DyPs (dye-decolorizing peroxidases) (EC 1.11.1.19) represent a new family of haem peroxidases widespread in bacteria, archaea, fungi and other micro-organisms. In the present study, we expressed A. auricula-judae DyP in E. coli, solved the crystal structure of the recombinant enzyme and several site-directed variants, and used PELE (Protein Energy Landscape Exploration) to describe the binding of its typical substrate RB19. The DyP structure is formed by two domains, each of them including an antiparallel four-stranded large β-sheet and two or three helices resulting in a ferredoxin-like fold (plus two additional β-strands). In spite of the obvious similarity between the two domains, only the C-terminal domain harbours a haem cofactor.

Among them, Tyr-147, Tyr337 and Trp-377 are solvent-exposed, but Trp-105 and Tyr-285 are buried into the protein making their interaction with the dye substrate more difficult. Aromatic residues were changed to serine in the simple W377S, Y147S and Y337S variants (the latter with low refolding yield). Moreover, most of the variants show crystal structures largely superimposable with that of WT DyP, except for the mutated residues. In contrast, similar Tyr-337 and Tyr-147 variants (and the double Y147F/Y337F variant) only slightly affected substrate oxidation, and did not remove the high-turnover site. However, this does not seem to be due to modification of Tyr-337 (or contiguous Tyr-147) since the enzyme activity was practically unaffected after site-directed mutagenesis of these two residues. Among the 65 DyP sequences compared, 58 include a tryptophan residue homologous with Trp-377, and 48 include a tyrosine residue homologous with Tyr-337 (whereas the neighbour Tyr-147 is only conserved in 14 sequences).

>MATSLNTIDIQGDILVGMHKQKQLFYFFAINDPATFKTHLASDIAPVVASVTQLSNVATQPLVALNIAFSNTGLLALGVTDNLGDSLFANGQAKDATSFKESTSSWVPQFAGTGIHGVIILASDTTDLIDQQVASIESTFGSSISKLSSLSASIRPGNEAGHEMFGFLDGIAQPAINGFNTPLPGQNIVDAGVIITGATNDPITRPSWAVGGSFLAFRQLEQLVPEFNKYLLDNAPAGSGSLQARADLLGARMVGRWKSGAPIDLTPTADDPALGADAQRNNNFTYSHAGFDLGSDQSHCPFSAHIRKTRPRADLGGSLTPPNLSAGANSIMRSGIPYGPEVTSAESASNTTTQERGLAFVAYQAQLSQGFHFLQQTWADNANFPPGKTPATVGLDPIIGQNNGQPRVVNGLLPSNSSASLSIPQFVVSHGGEYFFSPPISAIGGRLSA[2x]> MAYIKRVIIKGFKTYRNETIIDNFSPHQNVIIGSNGSGKSNFFAAIRFVLSDDYSNLKREERQGLIHQGSGGSVMSASVEIVFHDPDHSMILPSGVLSRGDDEVTIRRTVGLKKDDYQLNDRNVTKGDIVRMLETAGFSMNNPYNIVPQGKIVALTNAKDKERLQLLEDVVGAKSFEVKLKASLKKMEETEQKKIQINKEMGELNSKLSEMEQERKELEKYNELERNRKIYQFTLYDRELNEVINQMERLDGDYNNTVYSSESSKHPTSLVPRGSDITSDQLLQRLNDMNTEISGLKNVNKRAFENFKKFNERRKDLAERASELDESKDSIQDLIVKLKQQKVNAVDSTFQKVS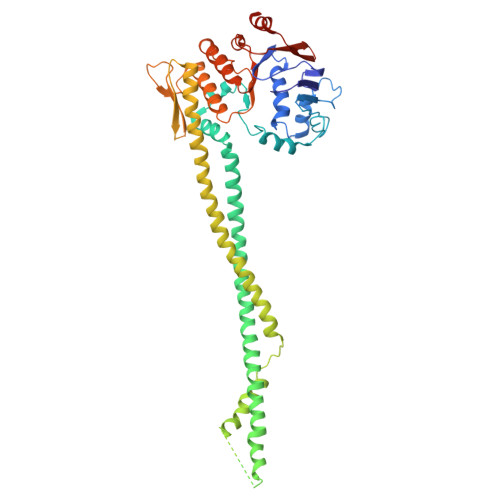ENFEAVFERLVPRGTAKLIIHRKNDNANDHDESIDVDMDAESNESQNGKDSEIMYTGVSISVSFNSKQNEQLHVEQLSGGQKTVCAIALILAIQMVDPASFYLFDEIDAALDKQYRTAVATLLKELSKNAQFICTTFRTDMLQVADKFFRVKYENKISTVIEVNREEAIGFIRGSNKFAEVWSHPQFEK> MKSPALQPLSMAGLQLMTPASSPMGPFFGLPWQQEAIHDNIYTPRKYQVELLEAALDHNTIVCLNTGSGKTFIAVLLTKELSYQIRGDFSRNGKRTVFLVNSANQVAQQVSAVRTHSDLKVGEYSNLEVNASWTKERWNQEFTKHQVLIMTCYVALNVLKNGYLSLSDINLLVFDECHLAILDHPYREIMKLCENCPSCPRILGLTASILNGKCDPEELEEKIQKLEKILKSNAETATDLVVLDRYTSQPCEIVVDCGPFTDRSGLYERLLMELEEALNFINDCNISVHSKERDSTLISKQILSDCRAVLVVLGPWCADKVAGMMVRELQKYIKHEQEELHRKFLLFTDTFLRKIHALCEEHFSPASLDLKFVTPKVIKLLEILRKYKPYERQQFESVEWYNNRNQDNYVSWSDSEDDDEDEEIEEKEKPETNFPSPFTNILCGIIFVERRYTAVVLNRLIKEAGKQDPELAYISSNFITGHGIGKNQPRNKQMEAEFRKQEEVLRKFRAHETNLLIATSIVEEGVDIPKCNLVVRFDLPTEYRSYVQSKGRARAPISNYIMLADTDKIKSFEEDLKTYKAIEKILRNKCSKSVDTGETDIDPVMDDDDVFPPYVLRPDDGGPRVTINTAIGHINRYCARLPSDPFTHLAPKCRTRELPDGTFYSTLYLPINSPLRASIVGPPMSCVRLAERVVALICCEKLHKIGELDDHLMPVGKETVKYEEELDLHDEEETSVPGRPGSTKRRQCYPKAIPECLRDSYPRPDQPCYLYVIGMVLTTPLPDELNFRRRKLYPPEDTTRCFGILTAKPIPQIPHFPVYTRSGEVTISIELKKSGFMLSLQMLELITRLHQYIFSHILRLEKPALEFKPTDADSAYCVLPLNVVNDSSTLDIDFKFMEDIEKSEARIGIPSTKYTKETPFVFKLEDYQDAVIIPRYRNFDQPHRFYVADVYTDLTPLSKFPSPEYETFAEYYKTKYNLDLTNLNQPLLDVDHTSSRLNLLTPRHLNQKGKALPLSSAEKRKAKWESLQNKQILVPELCAIHPIPASLWRKAVCLPSILYRLHCLLTAEELRAQTASDAGVGVRSLPADFRYPNLDFGWKKSIDSKSFISISNSSSAENDNYCKHSTIVPENAAHQGANRTSSLENHDQMSVNCRTLLSESPGKLHVEVSADLTAINGLSYNQNLANGSYDLANRDFCQGNQLNYYKQEIPVQPTTSYSIQNLYSYENQPQPSDECTLLSNKYLDGNANKSTSDGSPVMAVMPGTTDTIQVLKGRMDSEQSPSIGYSSRTLGPNPGLILQALTLSNASDGFNLERLEMLGDSFLKHAITTYLFCTYPDAHEGRL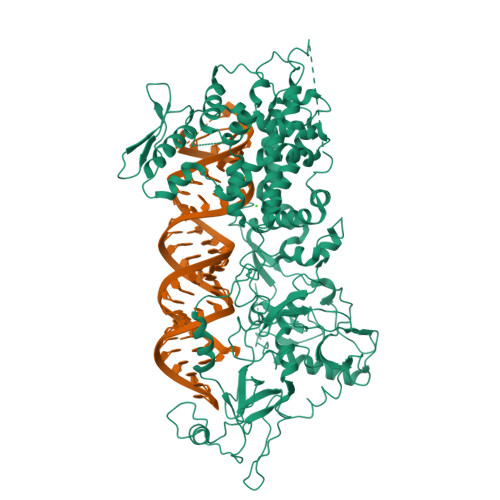SYMRSKKVSNCNLYRLGKKKGLPSRMVVSIFDPPVNWLPPGYVVNQDKSNTDKWEKDEMTKDCMLANGKLDEDYEEEDEEEESLMWRAPKEEADYEDDFLEYDQEHIRFIDNMLMGSGAFVKKISLSPFSTTDSAYEWKMPKKSSLGSMPFSSDFEDFDYSSWDAMCYLDPSKAVEEDDFVVGFWNPSEENCGVDTGKQSISYDLHTEQCIADKSIADCVEALLGCYLTSCGERAAQLFLCSLGLKVLPVIKRTDREKALCPTRENFNSQQKNLSVSCAAASVASSRSSVLKDSEYGCLKIPPRCMFDHPDADKTLNHLISGFENFEKKINYRFKNKAYLLQAFTHASYHYNTITDCYQRLEFLGDAILDYLITKHLYEDPRQHSPGVLTDLRSALVNNTIFASLAVKYDYHKYFKAVSPELFHVIDDFVQFQLEKNEMQGMDSELRRSEEDEEKEEDIEVPKAMGDIFESLAGAIYMDSGMSLETVWQVYYPMMRPLIEKFSANVPRSPVRELLEMEPETAKFSPAERTYDGKVRVTVEVVGKGKFKGVGRSYRIAKSAAARRALRSLKANQPQVPNS> PGSHMAEVKRKIEEELDRRAQPSDVGFLVKSEVLEALKPKIMKAAFMIRRAIFEGRPIILRHHADTDGYTAGVALETAIIPLIEKVAPDPEARWHLFKRRPSRAPFYELEDVLKDIIFMMEDHMRFGDELPLVVIVDNGGTTEDIPAYKRLKAYGVKIVVIDHHDPRDWISEDKAKVDEYVDVHVNPHHVKRGYYELTAGMLATEVARYINPEVEDRIKHLPAIAGTGDRSKAPEFYQYLEYAKEKGLDEEDLKKIAEVIDHEAFYWKFMDGRGIIEEILLITGNLQRHRMLVEGIYPEVKEKQEKVLKAVLPHVKSVVLPNGIRFNTIDVELYAPKFEYPSPGKLSGIIHDHFKEQYGEDSPILTLAYGPDFA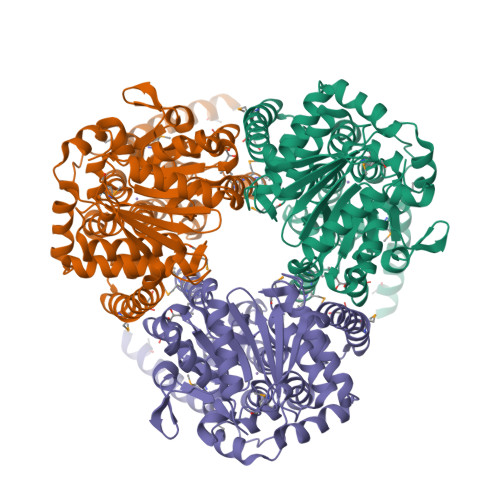VVRASDGMAKYNFDLNKIVKILAEKLPDAGVEGGGHSYAGSIKFFEGKRKEVLEAFAKEVLKLKAGE> GEIEFIESSKDAGFPVINTPSKTKLEPSVFHQVFEGNKEPAVLRSGDPRLKANFEEAIFSKYIGNVNTHVDEYMLEAVDHYAGQLATLDISTEPMKLEDAVYGTEGLEALDLTTSAGYPYVALGIKKRDILSKKTKDLTKLKECMDKYGLNLPMVTYVKDELRSIEKVAKGKSRLIEASSLNDSVAMRQTFGNLYKTFHLNPGVVTGSAVGCDPDLFWSKIPVMLDGHLIAFDYSGYDASLSPVWFACLKMLLEKLGYTHKETNYIDYLCNSHHLYRDKHYFVRGGMPSG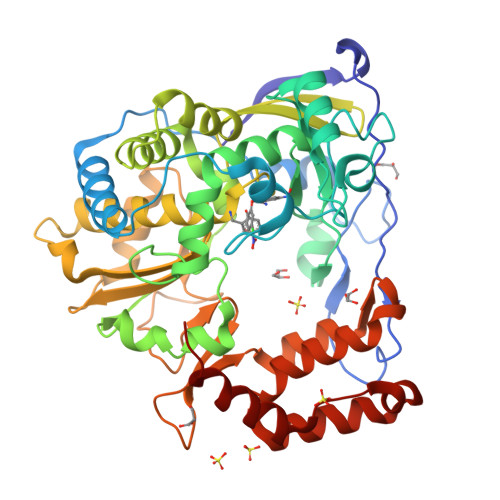CSGTSIFNSMINNIIIRTLMLKVYKGIDLDQFRMIAYGDDVIASYPWPIDASLLAEAGKGYGLIMTPADKGECFNEVTWTNATFLKRYFRADEQYPFLVHPVMPMKDIHESIRWTKDPKNTQDHVRSLCLLAWHNGEHEYEEFIRKIRSVPVGRCLTLPAFSTLRRKWLDSFHHHH> MPLAFCGTENHSAAYRVDQGVLNNGCFVDALNVVPHVFLLFITFPILFIGWGSQSSKVHIHHSTWLHFPGHNLRWILTFILLFVLVCEIAEGILSDGVTESRHLHLYMPAGMAFMAAITSVVYYHNIETSNFPKLLIALLIYWTLAFITKTIKFVKFYDHAIGFSQLRFCLTGLLVILYGMLLLVEVNVIRVRRYIFFKTPREVKPPEDLQDLGVRFLQPFVNLLSKGTYWWMNAFIKTAHKKPIDLRAIAKLPIAMRALTNYQRLCVAFDAQARKDTQSPQGARAIWRALCHAFGRRLILSSTFRILADLLGFAGPLCIFGIVDHLGKENHVFQPKTQFLGVYFVSSQEFLGNAYVLAVLLFLALLLQRTFLQASYYVAIETGINLRGAIQTKIYNKIMHMSTSNLSMGEMTAGQICNLVAIDTNQLMWFFFLCPNLWTMPVQIIVGVILLYYILGVSALIGAAVIILLAPVQYFVATKLSQAQRTTLEHSNERLKQTNEMLRGMKLLKLYAWESIFCSRVEVTRRKEMTSLRAFAVYTSISIFMNTAIPIAAVLITFVGHVSFFKESDLSPSVAFASLSLFHILVTPLFLLSSVVRSTVKALVSVQKLSEFLSSAEIREEQCAPREPAPQGQAGKYQAVPLKVVNRKRPAREEVRDLLGPLQRLAPSMDGDADNFCVQIIGGFFTWTPDGIPTLSNITIRIPRGQLTMIVGQVGCGKSSLLLATLGEMQKVSGAVFWNSNLPDSEGEDPSSPERETAAGSDIRSRGPVAYASQKPWLLNATVEENITFESPFNKQRYKMVIEACSLQPDIDILPHGDQTQIGERGINLSGGQRQRISVARALYQQTNVVFLDDPFSALDVHLSDHLMQAGILELLRDDKRTVVLVTHKLQYLPHADWIIAMKDGTIQREGTLKDFQRSECQLFEHWKTLMNRQDQELEKETVMERKASEPSQGLPRAMSSRDGLLLDEEEEEEEAAESEEDDNLSSVLHQRAKIPWRACTKYLSSAGILLLSLLVFSQLLKHMVLVAIDYWLAKWTDSALVLSPAARNCSLSQECDLDQSVYAMVFTLLCSLGIVLCLVTSVTVEWTGLKVAKRLHRSLLNRIILAPMRFFETTPLGSILNRFSSDCNTIDQHIPSTLECLSRSTLLCVSALTVISYVTPVFLVALLPLAVVCYFIQKYFRVASRDLQQLDDTTQLPLVSHFAETVEGLTTIRAFRYEARFQQKLLEYTDSNNIASLFLTAANRWLEVCMEYIGACVVLIAAATSISNSLHRELSAGLVGLGLTYALMVSNYLNWMVRNLADMEIQLGAVKRIHALLKTEAESYEGLLAPSLIPKNWPDQGKIQIQNLSVRYD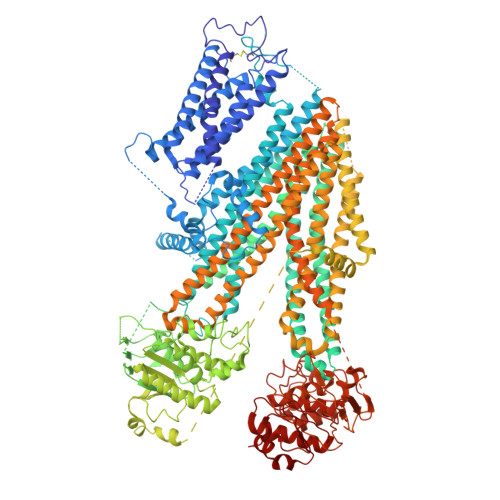SSLKPVLKHVNTLISPGQKIGICGRTGSGKSSFSLAFFRMVDMFEGRIIIDGIDIAKLPLHTLRSRLSIILQDPVLFSGTIRFNLDPEKKCSDSTLWEALEIAQLKLVVKALPGGLDAIITEGGENFSQGQRQLFCLARAFVRKTSIFIMDEATASIDMATENILQKVVMTAFADRTVVTIAHRVHTILSADLVMVLKRGAILEFDKPETLLSQKDSVFASFVRADK>[4x]MTIHKKGQAHWESDIKRGKGTVSTESGVLNQQPYGFNTRFEGEKGTNPEELIGAAHAACFSMALSLMLGEAGFTPTSIDTTADVS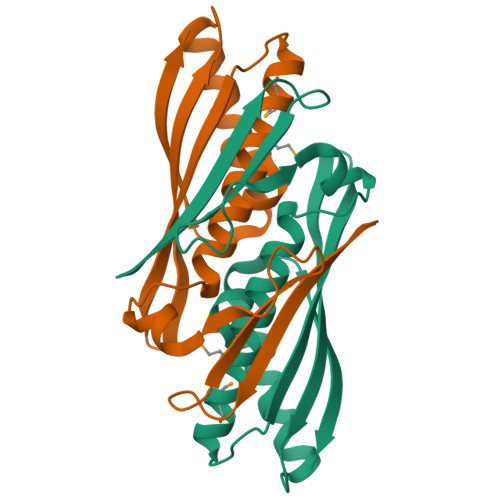LDKVDAGFAITKIALKSEVAVPGIDASTFDGIIQKAKAGCPVSQVLKAEITLDYQLKS>RVMDMKAPIKVYMTKKLLGVKPSTSVQEASRLMMEFDVGSLVVINDDGNVVGFFTKSDIIRRVIVPGLPYDIPVERIMTRNLITAN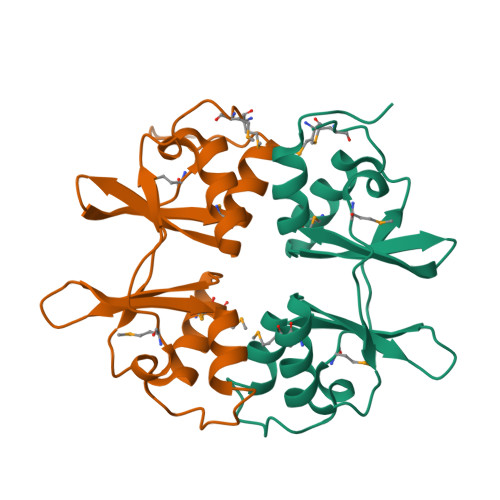VNTPLGEVLRKMAEHRIKHILIEEEGKIVGIFTLSDLLEASRRRLETAISAE[2x]> CPRFLKVKNWETDVVLTDTLHLKSTLETGCTEH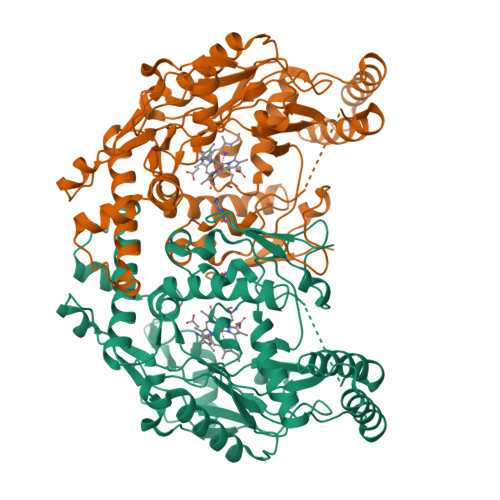ICMGSIMLPSQHTRKPEDVATKDQLFPLAKEFLDQYYSSIKRFGSKAHMDRLEEVNKEIESTSTYQLKDTELIYGAKHAWRNASRCVGRIQWSKLQVFDARDCTTAHGMFNYICNHVKYATNKGNLRSAITIFPQRTDGKHDFRVWNSQLIRYAGYKQPDGSTLGDPANVQFTEICIQQGWKAPRGRFDVLPLLLQANGNDPELFQIPPELVLEVPIRHPKFDWFKDLGLKWYGLPAVSNMLLEIGGLEFSACPFSGWYMGTEIGVRDYCDNSRYNILEEVAKKMDLDMRKTSSLWKDQALVEINIAVLYSFQSDKVTIVDHHSATESFIKHMENEYRCRGGCPADWVWIVPPMSGSITPVFFQEMLNYRLTPSFEYQPDPWNTHVWKG>MANVAVEFLVQNLMQLLRDNAELIVGVKDSAESLLQDLNDFNAFLKQTAKSRTENDVHKELVKKIKTVVNSAEDAIDKFVIEAKLHKDKGVGRFVDVKHYKRVYDVAGEIKTIRDKVKEIRLNNALDLQALQDEDQSAKGVQERKPPVVEEDDVVGFEEEADKVINRLLGGSSGLEVVPVVGMPGLGKTTLANKIYKHPDIGYQFFTRIWVYVSQSYRRRELFLNIISKFTRNTKQYHDMCEEDLADEIEDFLGKGGKYLIVLDDVWSPDAWERIRIAFPNNNKSNRILLTTRDSKVAKQCKQCIGIPHDLKFLTEDESWILLEKKVFHKDKCPPELELSGKSIAKKCNGLPLAIVVIAGALIGKGKTSREWKQVDESVGEHLINKDQPENCNKLVQLSYDRLSYDLKACFLYCGAFPGGFEIPAWKLIRLWIAEGFIQYKGHLSLECKAEDNLNDLINRNLVMVMQRTSDGQIKTCRLHDMLHEFCRQEAMKEENLFQEIKLGAEQYFPGKRELATYRRLCIHSSVLEFISTKPSGEHVRSFLSFSLKKIEMPSVDIPTIPKGFPLLRVFDVESINFSRFSKEFFQLYHLRYIAFSSDTIKIIPKHIGELWNIQTLIINTQQRSLDIQANIWNMERLRHLHTNSSAKLPVPVTPRSSKVPLVNQSLQTLSTIAPESCTEEVFARTPNLKKLGIRGKIAVLLEPNKSLLKNVKKLESLENLKLINDSSQTGKGLRLPPSYIFPTKLRKLSLVDTWLEWNDMSILGQMEHLEVLKLKENGFMGECWESVGGFCSLLVLWIERTDLVSWKASADHFPRLKHLVLICCDKLKEIPIGLADIRSFQVMELQNSTKTAAISARGIRDKKDKQTQEGTNNNGFKLSIFPPDL[6x]

NRCs are essential helper NLR (nucleotide-binding domain and leucine-rich repeat) proteins that execute immune responses triggered by sensor NLRs. Asterids—the largest group of flowering plants—have a complex immune receptor network composed of a multitude of sensor CC-NLRs that can signal redundantly via downstream helper MADA-type CC-NLRs, the NRCs (NLRs required for cell death). The N. benthamiana helper CC-NLR NbNRC2 exists as a homodimer at resting state and assembles into a higher-order oligomeric resistosome upon activation by Rx or other NRC-dependent sensor NLRs. NLRs typically exhibit a tripartite domain architecture consisting of an N-terminal signaling domain, a central nucleotide-binding (NB) and oligomerization module, and C-terminal superstructure-forming repeats.

We show that perception of the Potato virus X coat protein (PVX CP) by Rx triggers the formation of homohexameric NbNRC2 resistosomes, distinct from the previously reported pentameric assemblies formed by singleton CC-NLRs. We used an NbNRC2 variant with mutations in its N-terminal MADA motif (NbNRC2EEE), which was previously identified to abolish cell death induction without compromising receptor activation and oligomerization. The Rx-activated NbNRC2 oligomer contains six protomers that are assembled into a star-shaped resistosome. The α1 helices (residues 1 to 26), which carry the MADA consensus sequence, were not resolved in the NbNRC2 homohexamer, indicating their flexible nature. In the reconstruction, density was observed within the groove formed between the NB domain and HD1 domain of each protomer that is well modeled by a molecule of adenosine triphosphate (ATP). The ATP phosphate groups are coordinated by NB domain residues T189, T190, K188, and R293, and the adenine base is within a hydrophobic pocket bordered by F156 and V356. The most extensive interaction that stabilizes the central part of the resistosome is formed by the embedding of each HD1 domain within a concave surface of the adjacent protomer lined by the NB, WHD, and LRR regions. At the interface between NB domains, aspartate D239 and cysteine C241 from one protomer contact threonine T234 and asparagine N225 at distances of 3.3 and 4.4 Å, respectively, in the other protomer. By contrast, the two modules must undergo a rotation of approximately 180° with respect to each other to transition between the states. The α4 helix of NbNRC2 contains a bend near residue L126, which is at the end closest to the resistosome core.>[8x]MSLGDLEQKIIAMDLWHLALPVVSARDHGIGRVEGSCEIVVLRLVAEGGAEGFGEASPWAVFTGTPEASYAA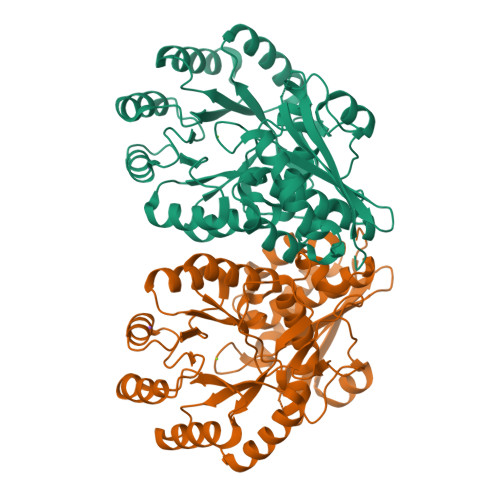LDRYLRPLVIGRRVGDRVAIMDEAARAVAHCTEAKAALDSALLDLAGRISNLPVWALLGGKCRDTIPLSCSIANPDFDADIALMERLRADGVGLIKLKTGFRDHAFDIMRLELIARDFPEFRVRVDYNQGLEIDEAVPRVLDVAQFQPDFIEQPVRAHHFELMARLRGLTDVPLLADESVYGPEDMVRAAHEGICDGVSIKIMKSGGLTRAQTVARIAAAHGLMAYGGDMFEAGLAHLAGTHMIAATPEITLGCEFYQASYFLNEDILETPFRVEAGQVIVPDGPGLGARADPEKLEHYAVRRSGEGHHHHHH> KMAFTLADRVTEEMLADKAALVVEVVEENYHDAPIVGIAVVNEHGRFFLRPETALADPQFVAWLGDETKKKSMFDSKRAAVALKWKGIELCGVSFDLLLAAYLLDPAQGVDDVAAAAKMKQ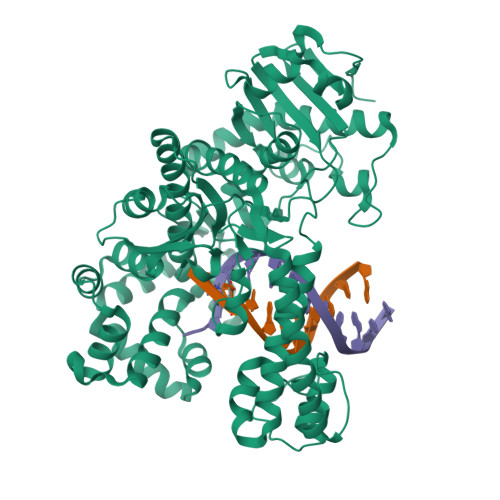YEAVRPDEAVYGKGAKRAVPDEPVLAEHLVRKAAAIWELERPFLDELRRNEQDRLLVELEQPLSSILAEMEFAGVKVDTKRLEQMGKELAEQLGTVEQRIYELAGQEFNINSPKQLGVILFEKLQLPVLKKTKTGYSTSADVLEKLAPYHEIVENILHYRQLGKLQSTYIEGLLKVVRPDTKKVHTIFNQALTQTGRLSSTEPNLQNIPIRLEEGRKIRQAFVPSESDWLIFAADYSQIELRVLAHIAEDDNLMEAFRRDLDIHTKTAMDIFQVSEDEVTPNMRRQAKAVNFGIVYGISDYGLAQNLNISRKEAAEFIERYFESFPGVKRYMENIVQEAKQKGYVTTLLHRRRYLPDITSRNFNVRSFAERMAMNTPIQGSAADIIKKAMIDLNARLKEERLQAHLLLQVHDELILEAPKEEMERLCRLVPEVMEQAVTLRVPLKVDYHYGSTWYDAK>MSTNEGSLWGGRFAGGPSDALAALSKSTHFDWVLAPYDLTASRAHTMVLFRAGLLTEEQRDGLLAGLDSLAQDVADGSFGPLVTDEDVHAALERGLIDRVGPDLGGRLRAGRSRNDQVAALFRMWLRDAVRRVATGVLDVVGALAEQAAAHPSAIMPGKTHLQSAQPILLAHHLLAHAHPLLRDLDRIVDFDKRAAVSPYGSGALAGSSLGLDPDAIAADLGFSAAADNSVDATAARDFAAEAAFVFAMIAVDLSRLAEDIIVWSSTEFGYVTLHDSWSTGSSIMPQKKNPDIAELARGKSGRLIGNLAGLLATLKAQPLAYNRDLQEDKEPVFDSVAQLELLLPAMAGLVASLTFNVQRMAELAPAGYTLATDLAEWLVRQGVPFRSAHEAAGAAVRAAEQRGVGLQELTDDELAAI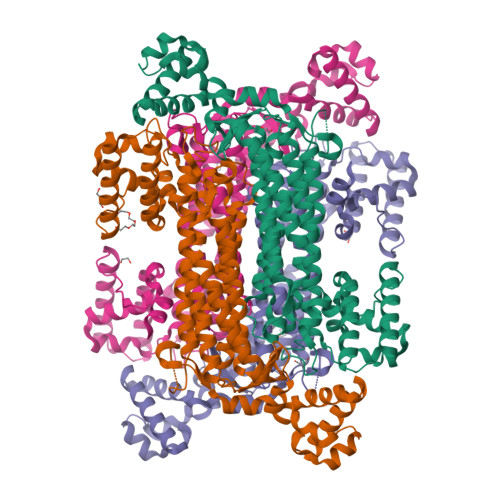SPELTPQVREVLTIEGSVSARDCRGGTAPGRVAEQLNAIGEAAERLRRQLVR[8x]>MNQNLLVTKRDGSTERINLDKIHRVLDWAAEGLHNVSISQVELRSHIQFYDGIKTSDIHETIIKAAADLISRDAPDYQYLAARLAIFHLRKKAYGQFEPPALYDHVVKMVEMGKYDNHLLEDYTEEEFKQMDTFIDHDRDMTFSYAAVKQLEGKYLVQNRVTGEIYESAQFLYILVAACLFSNYPRETRLQYVKRFYDAVSTFKISLPTPIMSGVRTPTRQFSSCVLIECGDSLDSINATSSAIVKYVSQRAGIGINAGRIRALGSPIRGGEAFHTGCIPFYKHFQ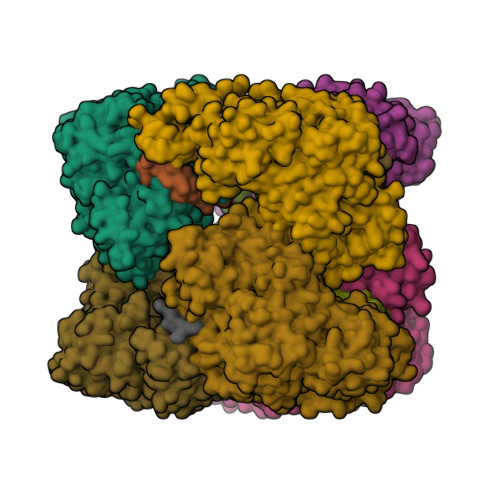TAVKSCSQGGVRGGAATLFYPMWHLEVESLLVLKNNRGVEGNRVRHMDYGVQINKLMYTRLLKGEDITLFSPSDVPGLYDAFFADQEEFERLYTKYEKDDSIRKQRVKAVELFSLMMQERASTGRIYIQNVDHCNTHSPFDPAIAPVRQSNLCLEIALPTKPLNDVNDENGEIALCTLSAFNLGAINNLDELEELAILAVRALDALLDYQDYPIPAAKRGAMGRRTLGIGVINFAYYLAKHGKRYSDGSANNLTHKTFEAIQYYLLKASNELAKEQGACPWFNETTYAKGILPIDTYKKDLDTIANEPLHYDWEALRESIKTHGLRNSTLSALMPSETSSQISNATNGIEPPRGYVSIKASKDGILRQVVPDYEHLHDAYELLWEMPGNDGYLQLVGIMQKFIDQSISANTNYDPSRFPSGKVPMQQLLKDLLTAYKFGVKTLFYQNTRDGAEDAQDDLVPSIQDDGCESGACKI[3x];>[4x]YLVGQIDSEVDTDDLSNFQL> SEKGNAKMIDFATLSKLKKK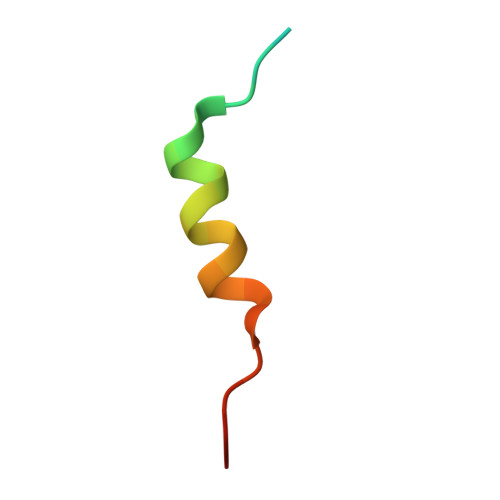YQIILDR> KRDLVQKLKILRQELSQQQPQAGHCRIEVSREEIFEESYRQVMKMRPKDLWKRLMIKFRGEEGLDYGGVAREWLYLLSHEMLN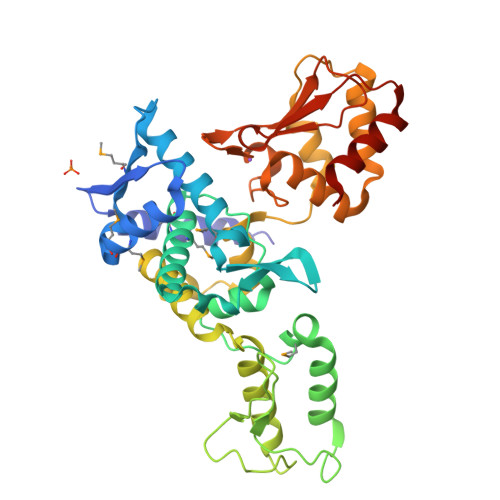PYYGLFQYSRDDIYTLQINPDSAVNPEHLSYFHFVGRIMGMAVFHGHYIDGGFTLPFYKQLLGKSITLDDMELVDPDLHNSLVWILENDITGVLDHTFCVEHNAYGEIIQHELKPNGKSIPVNEENKKEYVRLYVNWRFLRGIEAQFLALQKGFNEVIPQHLLKTFDEKELELIICGLGKIDVNDWKVNTRLKHCTPDSNIVKWFWKAVEFFDEERRARLLQFVTGSSRVPLQGFKALQGAAGPRLFTIHQIDACTNNLPKAHTCFNRIDIPPYESYEKLYEKLLTAIEETCGFAVE>[60x]AGGVGVSTGDFDNTTLWDFHEDGTATITCNSTRLVHLTRPDSLDYKIIPTQNNTAVQTVGHMMDDDNHTQVLTPWSLVDCNAWGVWLSPHDWQHIMNIGEELELLSLEQEVFNVTLKTATETGPPESRITMYNNDLTAVMMITTDTNNQLPYTPAAIRSETLGFYPWRPTVVPRWRYYFDWDRFLSVTSSSDQSTSIINHSSTQSAIGQFFVIETQLPIALLRTGDSYATGGYKFDCNKVNLGRHWQTTRSLGLPPKIEPPTSESALGTINQNARLAWRWGINDVHETNVVRPCTAGYNHPEWFYTHTLEGPAIDPAPPTSIPSNWGGGTPPDTRASSHNQQRITYNYNHGNKDENLNNFSLNPNNIEGSIINQGNFLSYEGNGQQINTTAGVAKNGETATSDPNLVRYMPNTYGVYTAVDHQGPVYPHGQIWDKQIHTDKKPELHCLAPFTCKNNPPGQMFVRIAPNLTDTFNATPTFSEIITYADFWWKGTLKMKIKLRPPHQWNIATVLGAAVNIGDAARFVPNRLGQLEFPVINGRIVPSTVY

The capsid also protects the genome enroute to the nucleus for uncoating and replication. This study determines the capsid structures of TuV and CuV using cryo-electron microscopy and image reconstruction (cryo-EM) at ~2.9 Å resolution and compares them to the recently determined structure of BuV and other protoparvoviruses toward functional annotation. The VP ORF encodes two overlapping structural proteins, VP1 and VP2, sixty copies of which assemble the T = 1 icosahedral capsid in an approximate 1:10 ratio, respectively. The individual VPs contain an eight-stranded (βB to βI) anti-parallel β-barrel motif, with the βBIDG sheet forming the interior surface of the capsid. The virus capsid plays a central role in the infection by the protoparvoviruses as it mediates the attachment of the virus to specific receptors on target cells.

Similarly, in 2014, TuV was detected in feces of a Tunisian child with unexplained diarrhea and TuV IgG in one child and one adult from Finland. However, one exception was the diffuse electron density observed for amino acids 533–534 exclusively in the TuV map located near the 2-fold depression where only weak density was present for the main chain at a sigma (σ) threshold of one preventing reliable placement of amino acid side chains. The less ordered state in this region of the TuV map could be the result of the presence of multiple smaller amino acids 531-GAAV-534 conferring flexibility to this loop. TuV exhibits the most extended 5-fold channel among the known capsid structures of all members of the Parvovirinae with a radial distance of ~135 Å from the center of the capsid. The extended channel in TuV is not the result of amino acid insertions in the loop, but is instead caused by a different structural configuration of the DE loops which runs more radially upright from the capsid surface, compared to MVMp where the apex of the loop is tilted. While clearly separated in the CuV capsid and completely merged into a single “spinwheel” in MVMp, the 3-fold protrusions in the TuV capsid displayed an intermediate phenotype, with the protrusion almost fused at the 3-fold axis. The intermediate phenotype seen in the TuV capsid is due to this loop being truncated by 6 amino acids compared to MVMp and adopting an alternate conformation. In TuV, both VR1 and VR3 display less variability to MVMp (local RMSD 1.6 – 2.2 Å) with no insertion or deletion in VR1 and a single amino acid deletion in VR3. The readouts from these arrays showed approximately the same average signal fluorescent intensity for both viruses with strong signals over background for TuV and weaker signals for CuV (~5-fold over background with large error bars). In the TuV array the 17 top glycan binders all represent SIA containing carbohydrates (14 highest are shown in Figure 6).> MDWRHKAVCRDEDPELFFPVGNSGPALAQIADAKLVCNRCPVTTECLSWALNTGQDSGVWGGMSEDERRALKRR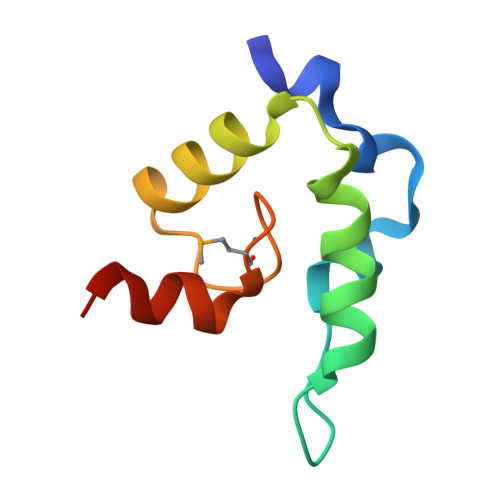NA> 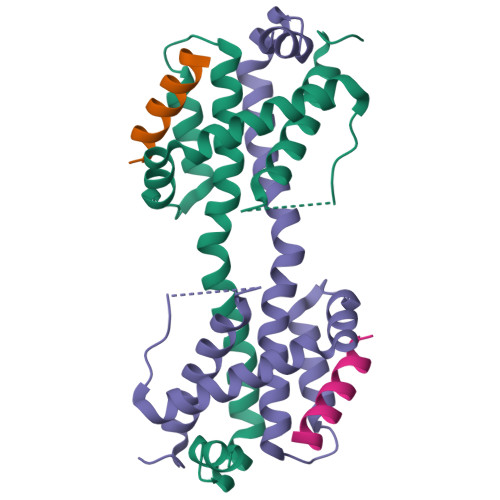MDGSGEQPRGGGPTSSEQIMKTGALLLQGFIQDRAGRMGGEAPELALDPVPQDASTKKLSESLKRIGDELDSNMELQRMIAAVDTDSPREVFFRVAADMFSDGNFNWGRVVALFYFASKLVLKALSTKVPELIRTIMGWTLDFLRERLLGWIQDQGGWDGLLSYFGSS;> DMRPEIWIAQELRRIGDEFN>[6x]RKNSDQEPSSKRKAQNRAAQRAFRKRKEDHLKALETQVVT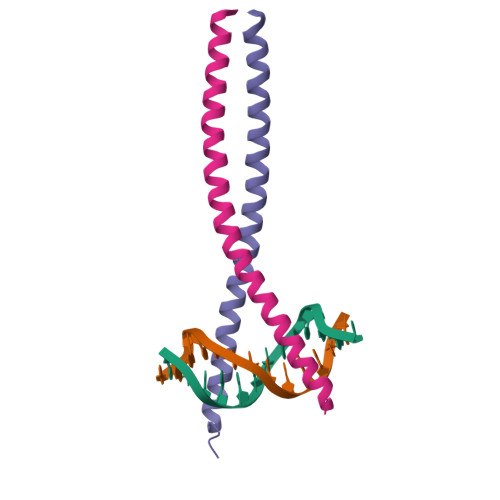LKELHSSTTLENDQLRQKVRQLEEELRILK> GSHMADKELKFLVVDDFSTMRRIVRNLLKELGFNNVEEAEDGVDALNKLQAGGYGFVISDWDMPNMDGLELL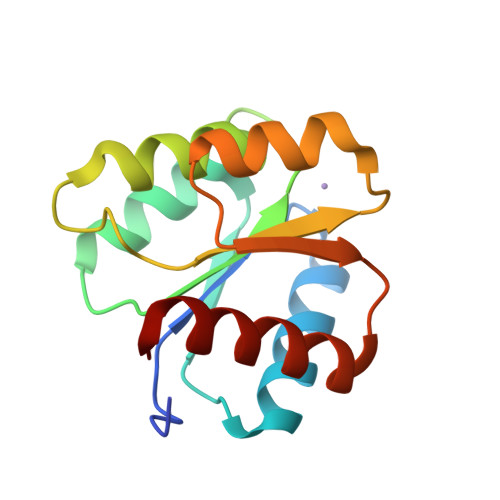KTIRADGAMSALPVLMVTARAKKENIIAAAQAGASGYVVKPFTAATLEEKLNKIFEKLGM>[2x]MKGKMAIVISTLNNPWFVVLAETAKQRAEQLGYEATIFDSQNDTAKESAHFDAIIAAGYDAIIFNPTDADGSIANVKRAKEAGIPVFCVDRGINARGLAVAQIYSDNYYGGVLAGEYFVKFLKEKYPDAKEIPYAELLGILSAQPTWDRSNGFHSVVDQYPEFKMVAQQSAEFDRDTAYKVTEQILQAH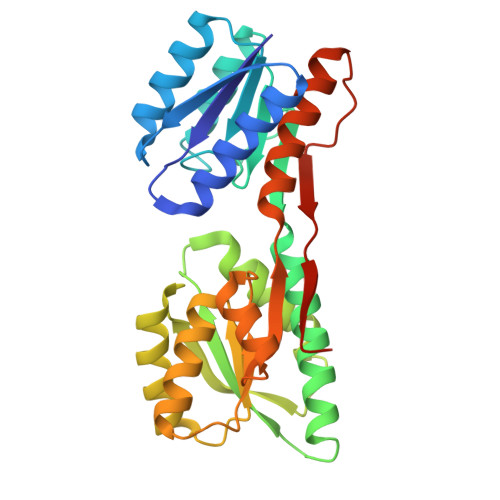PEIKAIWCGNDAMALGAMKACEAAGRTDIYIFGFDGAEDVINAIKEGKQIVATIMQFPKLMARLAVEWADQYLRGERSFPEIVPVTVELVTREGSHHHHHH> SSVVVDTNGQPVSNGADAYYLV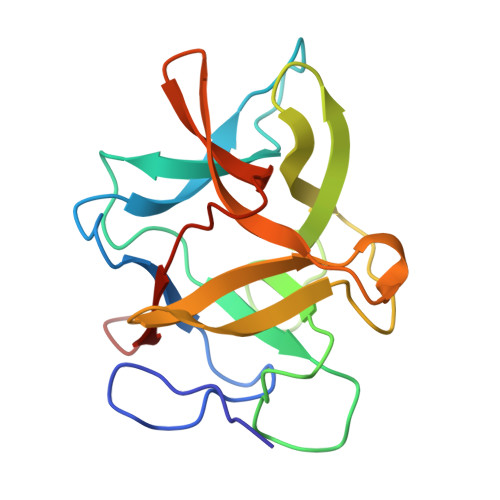PVSHGHAGLALAKIGNEAEPRAVVLDPHHRPGLPVRFESPLAINIIKESYFLNIKFGPSSSDSGVWDVIQQDPIGLAVKVTDTKSLLGPFKVEKEGEGYKIVYYPERGQTGLDIGLVHRNDKYYLAVKDGEPCVFKIRKATDE> MTESPTTHHGAAPPDSVATPVRPWSEFRLTPAEAAAAAALAARCAQRYDETDGPEFLLDAPVIAHELPKRLRTFMARARLDAWPHALVVRGNPVDDAALGSTPVHWRTARTPGSRPLSFLLMLYAGLLGDVFGWATQQDGRVVTDVLPIKGGEHTLVSSSSRQELGWHTEDAFSPYRADYVGLLSLRNPDGVATTLAGVPLDDLDERTLDVLFQERFLIRPDDSHLQVNNSTAQQGRVEFEGIAQAADRPEPVAILTGHRAAPHLRVDGDFSAP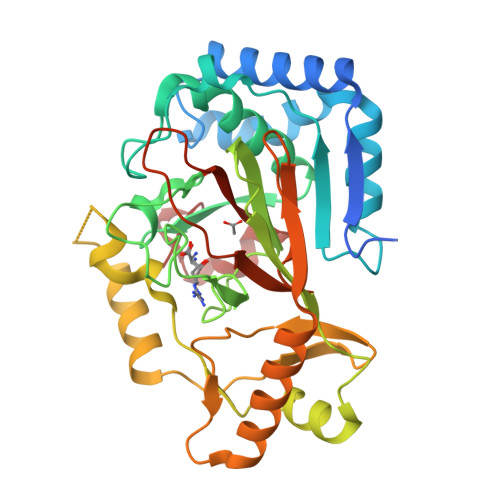AEGDEEAAAALGTLRKLIDASLYELVLDQGDVAFIDNRRAVHGRRAFQPRYDGRDRWLKRINITRDLHRSRKAWAGDSRVLGQR> ASQPPQVTVDKLKRLENDFGGRIGVYAIDTGSNKTFGYRANERFPLCSSFKGFLAAAVLSKSQQQEGLLNQRIRYDNRVMEPHSPVTEKQITTGMTVAELSAATLQYSDNGAANLLLEKLIGGPEGMTSFMRSIGDNVFRLDRWALELNSAIPGDDRD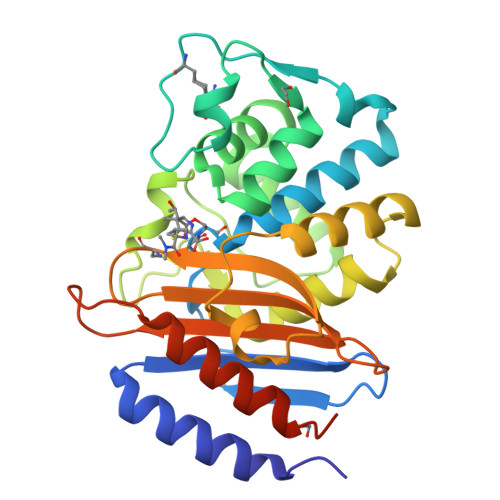TSTPKAVAESMQKLAFGNVLGLTERHQLMDWFKGNTTGGARIRASVPANWVVGDKTGTCGVYGTANDYAVIWPVAHAPIVLAVYTSKPDRNSKHSDAVIADASRIVLESFNIDALRMATGKSIGF> GGAGAVDEDDFIKAFTDVPSIQIYSSREL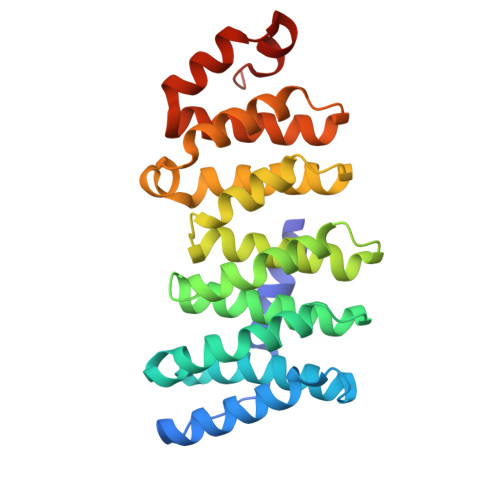EETLNKIREILSDDKHDWDQRANALKKIRSLLVAGAAQYDCFFQHLRLLDGALKLSAKDLRSQVVREACITVAHLSTVLGNKFDHGAEAIVPTLFNLVPNSAKVMATSGCAAIRFIIRHTHVPRLIPLITSNCTSKSVPVRRRSFEFLDLLLQEWQTHSLERHAAVLVETIKKGIHDADAEARVEARKTYMGLRNHFPGEAETLYNSLEPSYQKSLQTYLKS>[2x]GSSMDNQDGFILQQVKLSLDDPDSYLSSWNSNDASPCRWSGVSCAGDFSSVTSVDLSSANLAGPFPSVICRLSNLAHLSLYNNSINSTLPLNIAACKSLQTLDLSQNLLTGELPQTLADIPTLVHLDLTGNNFSGDIPASFGKFENLEVLSLVYNLLDGTIPPFLGNISTLKMLNLSYNPFSPSRIPPEFGNLTNLEVMWLTECHLVGQIPDSLGQLSKLVDLDLALNDLVGHIPPSLGGLTNVVQIELYN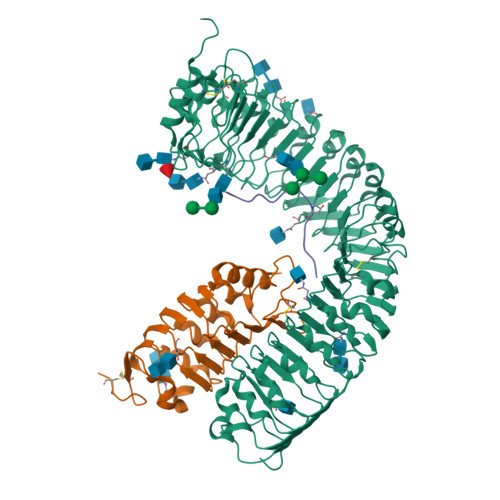NSLTGEIPPELGNLKSLRLLDASMNQLTGKIPDELCRVPLESLNLYENNLEGELPASIALSPNLYEIRIFGNRLTGGLPKDLGLNSPLRWLDVSENEFSGDLPADLCAKGELEELLIIHNSFSGVIPESLADCRSLTRIRLAYNRFSGSVPTGFWGLPHVNLLELVNNSFSGEISKSIGGASNLSLLILSNNEFTGSLPEEIGSLDNLNQLSASGNKFSGSLPDSLMSLGELGTLDLHGNQFSGELTSGIKSWKKLNELNLADNEFTGKIPDEIGSLSVLNYLDLSGNMFSGKIPVSLQSLKLNQLNLSYNRLSGDLPPSLAKDMYKNSFIGNPGLCGDIKGLCGSENEAKKRGYVLEGSENLYFQ;>GSSMASANLEGDALHTLRVTLVDPNNVLQSWDPTLVNPCTWFHVTCNNENSVIRVDLGNAELSGHLVPELGVLKNLQYLELYSNNITGPIPSNLGNLTNLVSLDLYLNSFSGPIPESLGKLSKLRFLRLNNNSLTGSIPMSLTNITTLQVLDLSNNRLSGSVPDNGSFSLFTPISFANNLDLCGPVTSHPCPLEGSLENLYFQ[2x];>YVLVPPSGPSMRHN[2x]> SNAADTVVQAGETVNGGTLTNHDNQIVLGTANGMTISTGLEYGPDNEANTGGQWIQNGGIANNTTVTGGGLQRVNAGGSVSDTVISAGGGQSLQGQAVNTTLNGGEQWVHEGGIATGTVINEKGWQAVKSGAMATDTVVNTGAEGGPDAENGDTGQTVYGDAVRTTINKNGRQIVAAEGTANTTVVYAGGDQTVHGHALDTTLNGGYQYVHNGGTASDTVVNSDGWQIIKEGGLADFTTVNQKGKLQVNAGGTATNVTLTQGGALVTSTAATVTGSNRLGNFTVE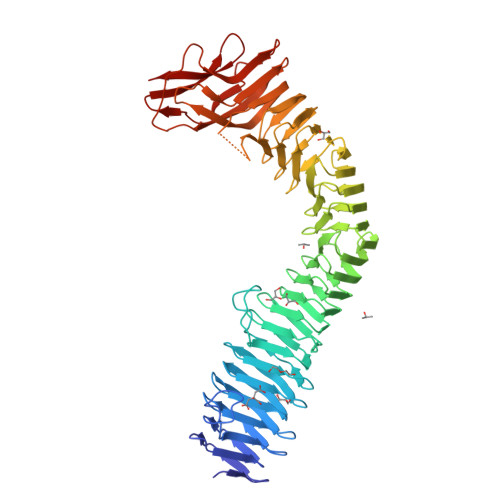NGNADGVVLESGGRLDVLEGHSAWKTLVDDGGTLAVSAGGKATDVTMTSGGALIADSGATVEGTNASGKFSIDGISGQASGLLLENGGSFTVNAGGLASNTTVGHRGTLTLAAGGSLSGRTQLSKGASMVLNGDVVSTGDIVNAGEIRFDNQTTPDAALSRAVAKGDSPVTFHKLTTSNLTGQGGTINMRVRLDGSNASDQLVINGGQATGKTWLAFTNVGNSNLGVATSGQGIRVVDAQNGATTEEGAFALSRPLQAGAFNYTLNRDSDEDWYLRSEN>MAEVIRSSAFWRSFPIFEEFDSETLCELSGI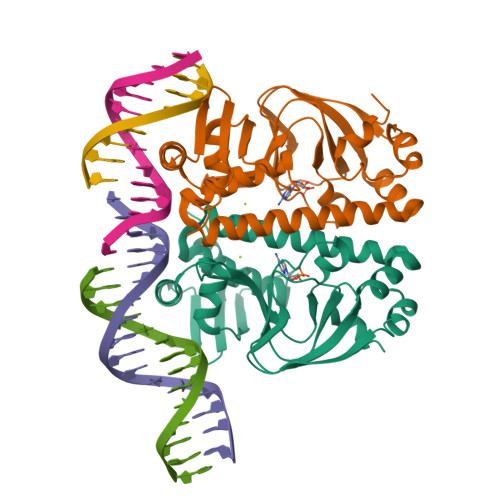ASYRKWSAGTVIFQRGDQGDYMIVVVSGRIKLSLFTPQGRELMLRQHEAGALFGEMALLDGQPRSADATAVTAAEGYVIGKKDFLALITQRPKTAEAVIRFLCAQLRDTTDRLETIALYDLNARVARFFLATLRQIHGSEMPQSANLRLTLSQTDIASILGASRPKVNRAILSLEESGAIKRADGIICCNVGRLLSIADPEEDLEHHHHHHHH[2x]> MSKSKVDNQFYSVEVGDSTFTVLKRYQNLKPIGSGAQGIVCAAYDAVLDRNVAIKKLSRPFQNQTHAKRAYRELVLMKCVNHKN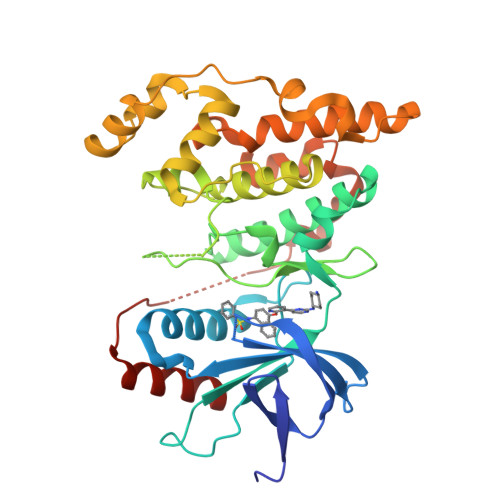IISLLNVFTPQKTLEEFQDVYLVMELMDANLCQVIQMELDHERMSYLLYQMLCGIKHLHSAGIIHRDLKPSNIVVKSDCTLKILDFGLARTAGTSFMMTPYVVTRYYRAPEVILGMGYKENVDIWSVGCIMGEMVRHKILFPGRDYIDQWNKVIEQLGTPCPEFMKKLQPTVRNYVENRPKYAGLTFPKLFPDSLFPADSEHNKLKASQARDLLSKMLVIDPAKRISVDDALQHPYINVWYDPAEVEAPPPQIYDKQLDEREHTIEEWKELIYKEVMNSE Glyceraldehyde-3-phosphate dehydrogenase (GAPDH) is an enzyme that catalyses the conversion of glyceraldehyde 3-phosphate to 1,3-bisphosphoglycerate using NAD+ as a cofactor and is known to be a moonlighting protein. Under normal cellular conditions, GAPDH primarily has a tetrameric conformation composed of four identical 35 kDa subunits. GAPDH consists of an NAD+-binding domain (residues 2–148 and 312–330), which is composed of α/β dinucleotide-binding folds or Rossmann folds, and a catalytic domain (residues 149–311), which is composed of eight antiparallel β-sheets with an α-helix and several short loops. An important region of GAPDH is the S-loop (residues 178–201), a long, winding region of the enzyme that is known to interact with some proteins.

In this study, the purification, crystallization and cryo­protection of Escherichia coli GAPDH (ecGAPDH) and the three-dimensional structure of trehalose-bound ecGAPDH are described. The GAPDH crystals were cryoprotected with a solution containing 15% of the disaccharide trehalose. The monomer contained 330 residues, one sulfate ion, one trehalose molecule and 171 water molecules. An electron-density map clearly indicated ordered tre­halose molecules bound to the protein. One trehalose molecule bound to ecGAPDH in the S-loop region. The S-loop region of GAPDH without NAD+ bound as a cofactor is very flexible and does not exhibit definite electron density. Despite the absence of NAD+, trehalose stabilized the S-loop of the enzyme. As a result, the electron-density map of the S-loop region of the protein was clear. The rotation of GAPDH also induced a conformational change in its active site. This suggests that the binding of trehalose to GAPDH induced a conformational change in its active site to prevent the binding of NAD+, although the NAD+- and trehalose-binding sites differ from one another. Although sucrose and maltose have similar structures to that of trehalose, these sugars did not bind to ecGAPDH and glycerol was not found, even though glycerol has previously been reported to be bound in GAPDH structures.

> MTIKVGINGFGRIGRIVFRAAQKRSDIEIVAINDLLDADYMAYMLKYDSTHGRFDGTVEVKDGHLIVNGKKIRVTAERDPANLKWDEVGVDVVAEATGLFLTDETARKHITAGAKKVVMTGPSKDNTPMFVKGANFDKYAGQDIVSNASCTTNCLAPLAKVINDNFGIIEGLMTTVHATTATQKTVDGPSHKDWRGGRGASQNIIPSSTGAAKAVGKVLPELNGKLTGMAFRVPTPNVSVVDLTVRLEKAATYEQIKAAVKAAAEGEMKGVLGYTEDDVVSTDFNGEVCTSVFDAKAGIALNDNFVKLVSWYDNETGYSNKVLDLIAHISK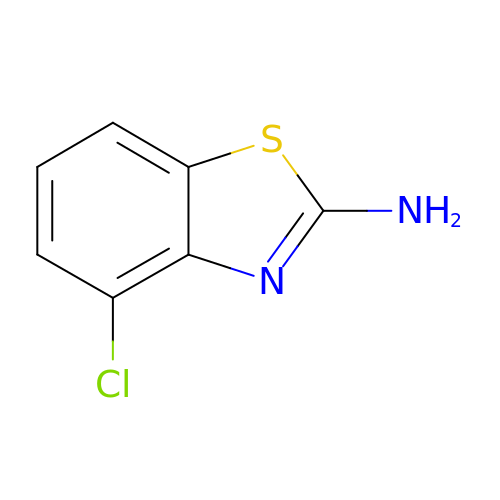4-chloro-1,3-benzothiazol-2-amine | C7 H5 Cl N2 S | OEQQFQXMCPMEIH-UHFFFAOYSA-N>[2x]TGSEIFLASKRAAITYDT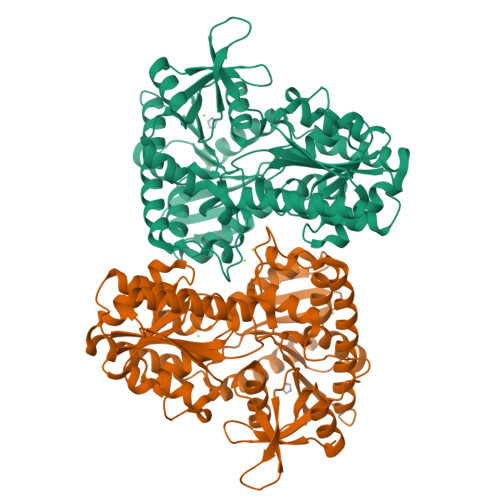DPATGEPRAWLAPGGTGNVVAEQAGVLNISWIASADSEDDRRASALNPDGVTMELHSGREILVRLIRHDPAVFRNVQNFMTANLMWAANNYGWDRWTQPSFGSDAREGWADFGRFTRDFADAILKSSAQSADPVYLVHDYQLVGVPALLREQRPDAPILLFVHIPWPSADYWRILPKEIRTGILHGMLPATTIGFFADRWCRNFLESVADLLPDARIDREAMTVEWRGHRTRLRTMPLGYSPLTLDGRNPQLPEGIEEWADGHRLVVHSGRTDPIKNAERAVRAFVLAARGGGLEKTRMLVRMNPNRLYVPANADYVHRVETAVAEANAELGSDTVRIDNDNDVNHTIACFRRADLLIFNSTVDGQNLSTFEAPLVNERDADVILSETCGAAEVLGEYCRSVNPFDLVEQAEAISAALAAGPRQRAEAAARRRDAARPWTLEAWVQAQLDGLAADHAARTATAERFDTAPAVSTRADL> AQPDIKFASKEYGVTIGESRIIYPLDAAGVMVSVKNTQDAPVLIQSRIYDENKEKESEDPFVVTPPLFRLDAKQQNSLRIAQAGGVFPRDKESLKWLCVKGIPPKDEDIWVDDATNKQKFNPDKDVGVFVQFAINNCIKLLVRPNELKGTPIQFAENLSWKVDGGKLIAENPSPFYMNIGELTFGGKSIPSHYIPPKSTWAFDLPKGLAGAR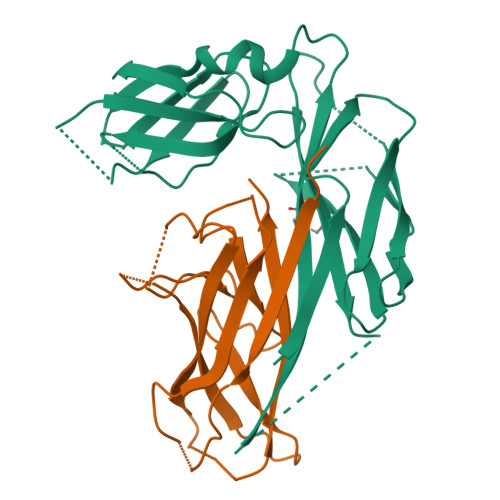NVSWRIINDQGGLDRLYSKNVTL;> ADLTASTTATATLVEPARITLTYKEGAPITIMDNGNIDTELLVGTLTLGGYKTGTTSTSVNFTDAAGDPMYLTFTSQDGNNHQFTTKVIGKDSRDFDISPKVNGENLVGDDVVLATGSQDFFVRSIGSKGGKLAAGKYTDAVTVTVSNQ>[2x]TRDRVPTYQYNMNFEKLGKCIIINNKNFDKVTGMGVRNGTDKDAEALFKCFRSLGFDVIVYNDCSCAKMQDLLKKASEEDHTNAACFACILLSHGEENVIYGKDGVTPIKDLTAHFRGARCKTLLEKPKLFFIQACRGTELDDGIQAD;>SGPINDTDANPRYKIPVEADFLFAYSTVPGYYSWRSPGRGSWFVQALCSILEEHGKDLEIMQILTRVNDRVARHFESQSDDPHFHEKKQIPCVVSMLT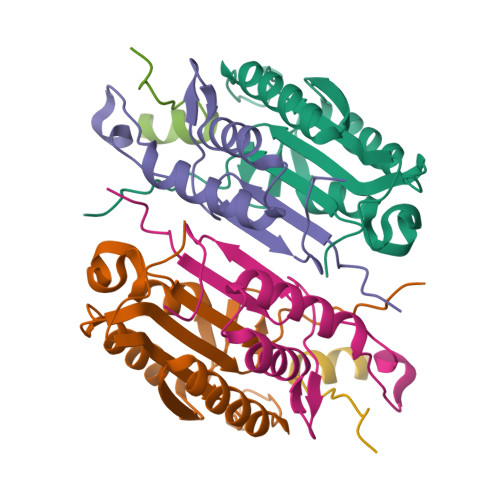KELYFSQ[2x];>[2x]RDHFALDRPSETHADYLLRTGQVVDISDTIYPRNPAMYCEEARLKSFQNWPDYAHLTPRELASAGLYYTGIGDQVQCFCCGGKLKNWEPCDRAWSEHRRHFPNCFFVLGRNLNIRSE>[3x]MVDVIALGEPLIQFNSFNPGPLRFVNYFEKHVAGSELNFCIAVVRNHLSCSLIARVGNDEFGKNIIEYSRAQGIDTSHIKVDNESFTGIYFIQRGYPIPMKSELVYYRKGSAGS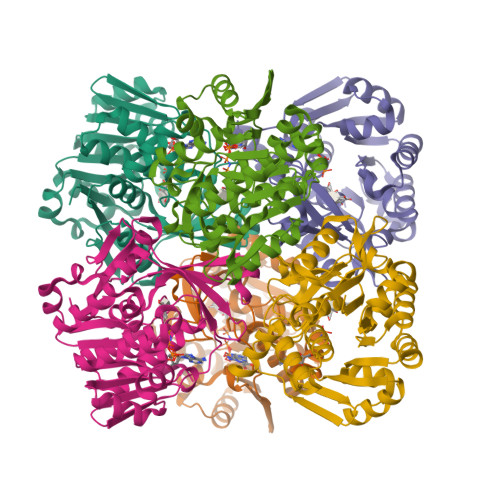RLSPEDINENYVRNSRLVHSTGITLAISDNAKEAVIKAFELAKSRSLDTNIRPKLWSSLEKAKETILSILKKYDIEVLITDPDDTKILLDVTDPDEAYRKYKELGVKVLLYKLGSKGAIAYKDNVKAFKDAYKVPVEDPTGAGDAMAGTFVSLYLQGKDIEYSLAHGIAASTLVITVRGDNELTPTLEDAERFLNEFKT>[2x]MSENLKDEILEKYIPKTKKTRSGHIVIKTEETPNPEIVANTRTVPGIITARGCAYAGCKGVVMGPIKDMVHITHGPIGCSFYTWGGRRFKSKPENGTGLNFNEYVFSTDMQESDIVFGGVNKLKDAIHEAYEMFHPAAIGVYATCPVGLIGDDILAVAATASKEIGIPVHAFSCEGYKGVSQSAGHHIANNTVMTDIIGKGNKEQKKYSINVLGEYNIGGDAWEMDRVLEKIGYHVNATLTGDATYEKVQNADKADLNLVQCHRSINYIAEMMETKYGIPWIKCNFIGVDGIVETLRDMAKCFDDPELTKRTEEVIAEEIAAIQDDLDYFKEKLQGKTACLYVGGSRSHTYMNMLKSFGVDSLVAGFEFAHRDDYEGREVIPTIKIDADSKNIPEITVTPDEQKYRVVIPEDKVEELKKAGVPLSSYGGMMKEMHDGTILIDDMNHHDMEVVLEKLKPDMFFAGIKEKFVIQKGGVLSKQLHSYDYNGPYAGFRGVVNFGHELVNGIYTPAWKMITPPWKKASSESKVVVGGEA;>MLDATPKEIVERKALRINPAKTCQPVGAMYAALGIHNCLPHSHGSQGCCSYHRTVLSRHFKEPAMASTSSFTEGASVFGGGSNIKTAVKNIFSLYNPDIIAVHTTCLSETLGDDLPTYISQMEDAGSIPEGKLVIHTNTPSYVGSHVTGFANMVQGIVNYLSENTGAKNGKINVIPGFVGPADMREIKRLFEAMDIPYIMFPDTSGVLDGPTTGEYKMYPEGGTKIEDLKDTGNSDLTLSLGSYASDLGAKTLEKKCKVPFKTLRTPIGVSATDEFIMALSEATGKEVPASIEEERGQLIDLMIDAQQYLQGKKVALLGDPDEIIALSKFIIELGAIPKYVVTGTPGMKFQKEIDAMLAEAGIEGSKVKVEGDFFDVHQWIKNEGVDLLISNTYGKFIAREENIPFVRFGFPIMDRYGHYYNPKVGYKGAIRLVEEITNVILDKIERECTEEDFEVVR[2x]

Biological nitrogen fixation is the process of reducing atmos­pheric dinitrogen to a biologically available form, such as ammonia, catalyzed by the enzyme nitrogenase found in certain bacteria and archaea. Nitrogenase is composed of two metalloprotein components, the molybdenum–iron (MoFe) protein and the iron (Fe) protein in the well characterized molybdenum nitrogenase system. The MoFe protein forms a dimer of heterodimers (α2β2) containing two complex metalloclusters in each αβ heterodimer: the [8Fe–7S] P cluster bridging the α-subunit and β-subunit and the [7Fe–Mo–9S–C–homocitrate] FeMo cofactor buried inside the α-subunit. The FeMo cofactor provides the active site for substrate reduction, while the P cluster is believed to serve as a relay for electron transfer from the [4Fe–4S] cluster of the Fe protein to the FeMo cofactor.

The X-ray crystal structure of the nitrogenase MoFe protein from Clostridium pasteurianum (Cp1) has been determined at 1.08 Å resolution by multiwavelength anomalous diffraction phasing. Cp1 and the ortholog from Azotobacter vinelandii (Av1) represent two distinct families of nitrogenases, differing primarily by a long insertion in the α-subunit and a deletion in the β-subunit of Cp1 relative to Av1. With the exceptions of the long insertion (residues 376–429 in Cp1) and deletion (residues 1–47 in Av1) in the α-subunit and β-subunit, respectively, the overall structures of the Cp1 and Av1 folds are similar and can be superimposed with a root-mean-square deviation (r.m.s.d.) of the main chain of 0.92 Å for 1554 aligned residues (78% of the Cp1 sequence). The long insert (residues 376–429) in the α-subunit of Cp1 adopts an irregularly structured loop involving residues 386–408 that is flanked by a short helix on each end. The long α-subunit insertion loop occludes the presumed Fe protein docking surface on Cp1 with few contacts to the remainder of the protein. This makes it plausible that this loop is repositioned to open up the Fe protein docking surface for complex formation. Our analysis confirms that the metal centers, the FeMo cofactor and the P cluster metallocluster, and the Fe16 mononuclear metal-binding site are essentially identical in Av1 and Cp1. Electron-density analysis and model fitting indicate that the P cluster in Cp1 corresponds to a mixture of the PN and POX conformations, as was also observed in the 1.0 Å resolution Av1 structure. The side chain of Serβ141 in Cp1 also shows two alternative conformations with the hydroxyl-group O atoms positioned 2.1 Å apart, correlated with the alternative conformations of Fe6 in the P cluster. We found, using either method, that Fe16 in Cp1 is about half occupied with little variation between crystals.> MTEQRPLTIALVAGETSGDILGAGLIRALKEHVPNARFVGVAGPRMQAEGCEAWYEMEELAVMGISESSGRSRRSSHIRADLTKRFGELKPDVFVGIDAPDFNITLEGNLKKQGIKTIHYVSPSVWAWRQKRVFKIGRATDLVLAFLPFEKAFYDKYNVPCRFIGHTMADAMPLDPDKNAARDVLGIPHDAHCLALLPGSRGAEVESLSADFLKTAQ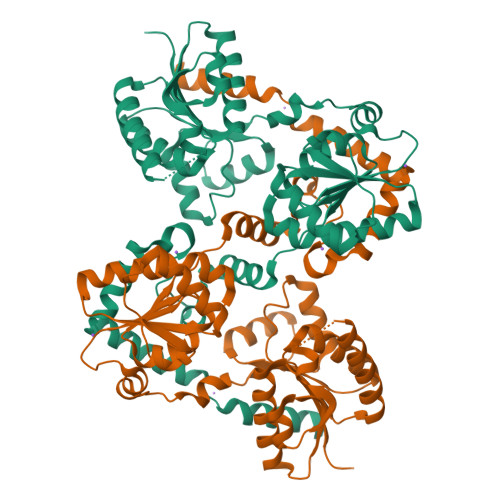LLRQTYPDLEIVVPLVNAKRREQFERIKAEVAPDLSVHLLDGMGREAMVASDAALLASGTAALECMLSKCPMVVGYRMKPFTFWLAKRLVKTDYVSLPNLLAGRELVKELLQEECEPQKLAAALLPLLANGKTSHAMHDTFRELHQQIRCNADEQAAQAVLELAQ> XTSFLEY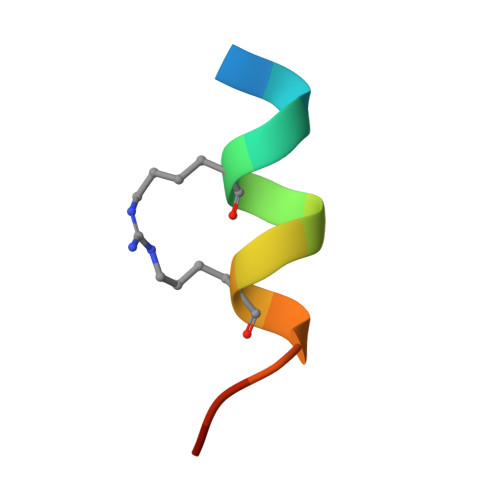WRLLSPX> ETGRNLPKQLTQATQVAWSGPPPGFAKCPGGQVVILGFAMHLNFKEPGTDNFRIISCPPGREKCDGVGTASSETDEGRIYILCGEEPINEIQQVVAESPAHAGASVLEASCPDETVVVGGFGISVRGGSDGLDSFSIESCTTGQTICTKAPTRGSEKNFLWMMCVDKQYPGLRELVNVAELGSHGNANKRAVNSDGNVDVKCPANSSIVLGYVMEAHTNMQFVRDKFLQCPENASECKMTGKGVDHGMLWLFDRHALFGWIICKTVNEGTKHHH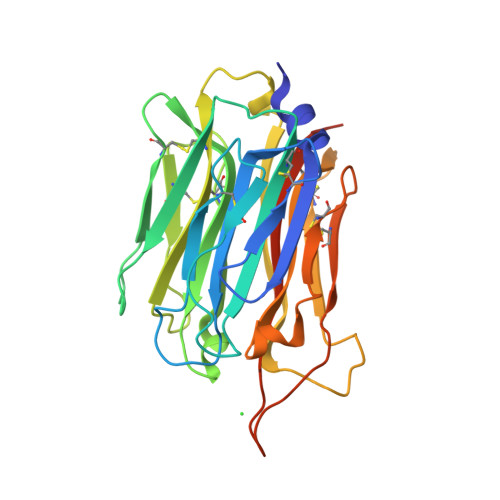HHH> GSLVLSELSQGLAVELMERVMMEFVRETCSQELKNAVETDQRVRVARCCEDVCAHLVDLFLV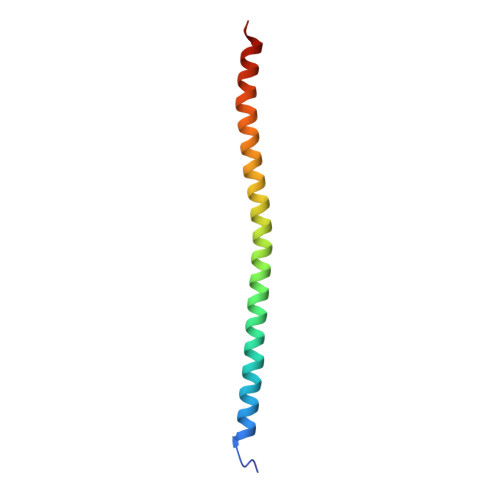EEIFQTAKETLQE>GSHMASQDNDDIFGNDSPEVPIFRKNLEKFKFSKGDGIKFSNTTFHIYEATRNYVTIHILKKYATAELMEFMHTRHD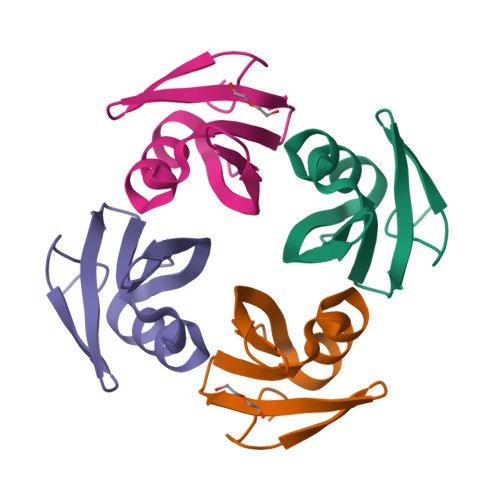AVYIGPILEWTDGVHLTFRRKS[4x]> SMVEISALPLRDLDYIKLATDQFGCRFLQKKLETPSESNMVRDLMYEQIKPFFLDLILDPFGNYLVQKLCDYLTAEQKTLLIQTIYPNVFQISINQYGTRSLQKIIDTVDNEVQIDLIIKGFSQEFTSIEQVVTLINDLNGNHVIQKCIFKFSPSKFGFIIDAIVEQNNIITISTHKHGCCVLQKLLSVCTLQQIFKISVKIVQFLPGLINDQFGNYIIQFLLDIKELDFYLLAELFNRLSNELCQLSCLKFSSNVVEKFIKKLFRIITGFIVNNNGGASQRTAVASDDVINASMNILLTTIDIFTVNLNVLIRDNFGNYALQTLLDVKNYSPLLAYNKNSNAIGQNSSSTLNYGNFCNDFSLKIGNLIVLTKELLPSIKTTSYAKKIKLKVKAYAEATG

PUF proteins are exemplary mRNA regulators. Puf5p is a broad regulator of RNAs in S. cerevisiae, binding to >1,000 RNA targets, constituting ∼16% of the transcriptome. The protein scaffold comprises eight α-helical repeats flanked by a short N-terminal sequence and a C-terminal helix (R8′). To understand how Puf5p accommodates a wide range of target site lengths, we determined crystal structures of the Puf5p RNA-binding domain bound to RNAs of 9–12 nt, including the recognition sequences in SMX2 (9 nt, 2.35-Å resolution), MFA2 (10 nt, 2.15-Å resolution), AAT2 (11 nt, 2.5-Å resolution) and AMN1 (12 nt, 2.8-Å resolution) mRNAs (sites of 8 nt did not crystallize).

Puf5p binds to the 9-nt SMX2 RNA site by recognizing all but the central fifth base. Bases 1–4 and 6–9 are each recognized by a PUF repeat. However, the fifth base, C5, lies in an atypical conformation, in which the plane of the base is parallel to the axis of the protein, within van der Waals bonding distance of the side chain of Cys381 in repeat 5. The ribose rings of C5 and U6 adopt C2′-endo conformations to accommodate positioning base C5. We refer to this conformation as ‘5-parallel'. Repeat 5 also lacks a large side chain capable of stacking with RNA bases and lies opposite several of the atypical RNA conformations (5-parallel, 5-stacked and triple-stacked). Recognition of the 5′-UGUA and 3′-UA elements by repeats 5–8 and 1–2, respectively, are identical in all structures.>MSIRDEALLVGTKVTTKAGDKNIENITLEDEVLQFDMNTKDFSYTNPTKTQKVIRDEIYHFEGAGFDQKVSPNHRMIYEQGGEIKECLAKDFEPSEDKYFIIVEGSHMQIKRIKSTDVKITHTKLDEPTEFHA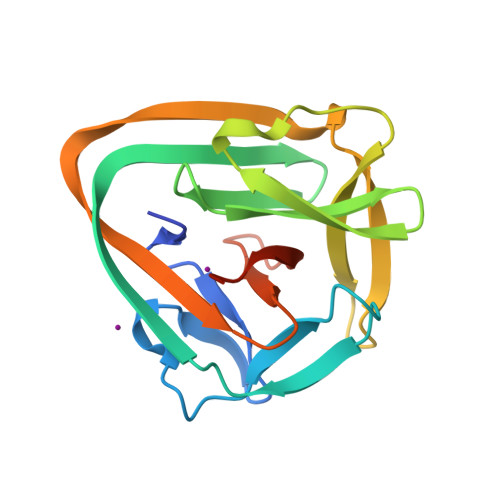LSVPGKSFVVTDEHGNRSVTGASMHVEGKLGG[2x]2-{(3S)-3-[(benzylsulfonyl)amino]-2-oxopiperidin-1-yl}-N-{(2S)-1-[(3S)-1-carbamimidoylpiperidin-3-yl]-3-oxopropan-2-yl}acetamide | C23 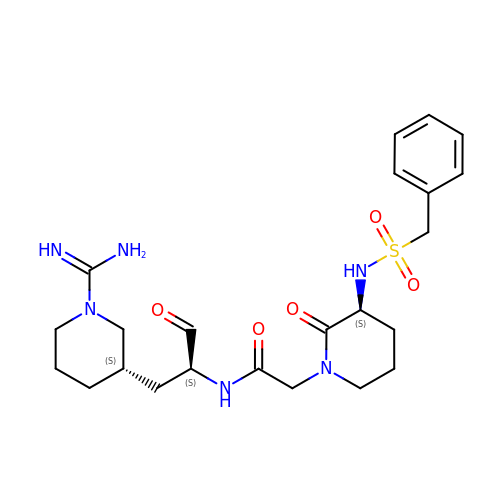H34 N6 O5 S | DATYERRDSFNBDN-UFYCRDLUSA-N> MSGSHHHHHHSGSMSPSPIEEQATRLLKEVPLIDGHNNFPYMIRGWFRNDINGQDAHLYDMPIGQTDLQRLQKGLLGGQFWSAFVPCPKNPDKEVGSLEALRQTLQQLDVIHRLIERHPTILQFADSAASIWSSFR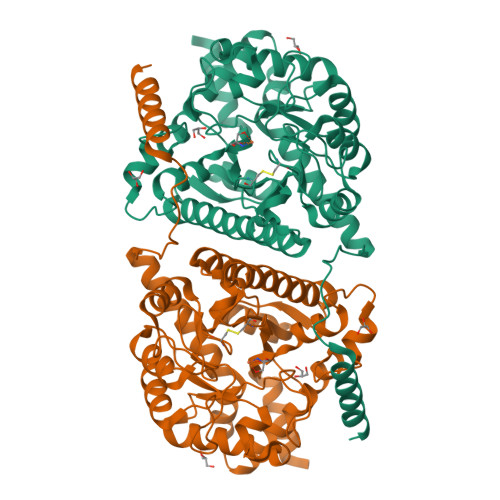AGRVASLIGIEGLHQIADSVSALRMLHRLGVRYVTLTHNCHNAFADAATVSPELHGGLSRKGERLIRELNRMGMMIDLSHTSHEAQTQALRLSRAPVIYSHSSIYSLRAHARNVTDENLHLLHRNRGVVMICFLRELLASEADQATLAHVIDHIIYAGTRIGYEHVGIGSDFDGMLRGPDGLHDVSCYPALVAGLLERGVSEEDVKRVMGLNVIRVLEEVERVAAELQGAGEECLCDELDEVWNEDIKEQLTRERERVRKLGPQK> DS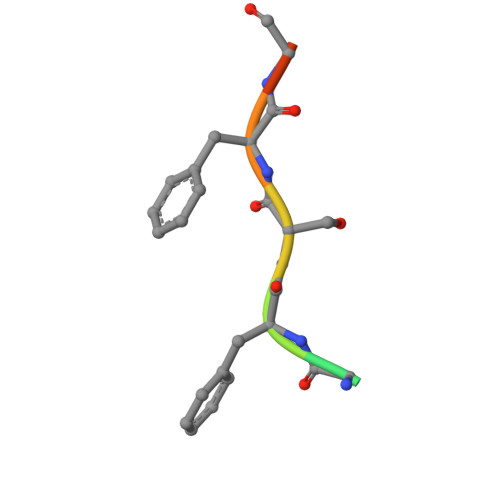GFSFGSK>MPNYKLLYFNMRGRAEIIRYIFAYLDIKYEDHRIEQADWPKIKPTLPFGKIPVLEVEGLTLHQSLAIARYLTKNTDLAGKTELEQ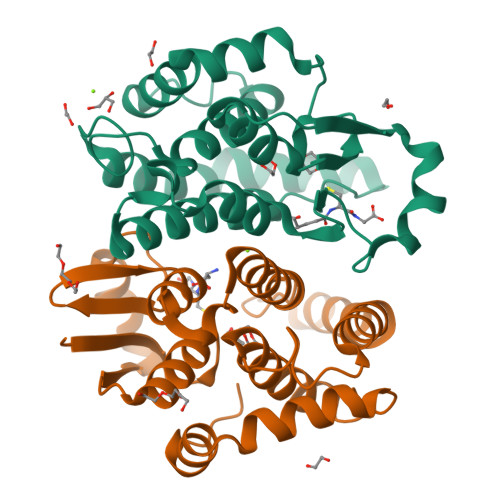CQVDAVVDTLDDFMSLFPWAEENQDLKERTFNDLLTRQAPHLLKDLDTYLGDKEWFIGNYVTWADFYWDICSTTLLVLKPDLLGIYPRLVSLRNKVQAIPAISAWILKRPQTKL[2x]Spiroplasma virus 4 (SpV4) is a bacteriophage of the Microviridae, which packages circular ssDNA within non-enveloped T = 1 icosahedral capsids. ORF1 expresses viral protein 1 (VP1), with a molecular weight of ~62 kDa, which is the major capsid protein. Lastly, VP8 encodes for an arginine–lysine-rich polypeptide that is analogous to the J-protein of phiX174 and is important for DNA packaging. A striking feature of the SpV4 capsid is the mushroom-like protrusions at the 3-fold axes, which is common among all members of the subfamily Gokushovirinae.

In this study, the capsid structures of genome-containing and empty SpV4 virions were determined to 2.5 and 3.0 Å resolution, respectively, using cryo-electron microscopy (cryo-EM) and three-dimensional (3D) image reconstruction. The observed order in the density map for the full capsids started at methionine 5 to the C-terminal isoleucine 553. An exception to the structural ordering is the surface loop at the 3-fold symmetry axis comprising aa230–291, for which only diffuse density was observed, preventing the placement of the polypeptide sequence. The SpV4 VP1 structure consists of a core, eight-stranded, anti-parallel β-barrel motif, with β-BIDG forming the inner surface of the capsid and the β-CHEF situated above β-BIDG. The EF-loop subloops are primarily situated around the 2-fold symmetry axis of the capsid surface, with the exception of the subloop EF4 that forms the mushroom-like protrusion at the 3-fold symmetry axis. The HI subloops occupy the space between the icosahedral symmetry axes, whereas the FG loop forms the channel around the 5-fold symmetry axes. The 5-fold symmetry axis showed a pore with a diameter of 4.5 Å at its narrowest point. The VP8, DNA-binding protein was observed in the interior of both genome-filled and empty SpV4 capsids. For this short, highly positively charged protein with a calculated pI of 12.9, structural order was observed for aa9–38. The N-terminal eight amino acids were not ordered but based on the first ordered residue, they should be located near the 5-fold axis. Its C-terminal phenylalanine 38 is buried inside the capsid core, in a very highly hydrophobic region near the 2-fold symmetry axis between β-CHEF, αA, and αB.

>[60x]MRRKVKNTKRHQWRLTHSARSIKRANIMPSNPRGGRRF;>[60x]MKKKMSKLNARVHDFSMFKGNHIPRSKIHIPHKTIRAFNVGEIIPIYQTPVYPGEHIKMDLTSLYRPSTFIVPPMDDLIVDTYAFAVPWRIVWKDLEKFFGENSDSWDVKNAPPVPDIVAPSGGWDYGTLADHFGITPKVPGIRVKSLRFRAYAKIINDWFRDQNLSSECALTLDSSNSQGSNGSNQVTDIQLGGKPYIANKYHDYFTSCLPAPQKGAPTTLNVGGMAPVTTKFRDVPNLSGTPLIFRDNKGRTIKTGQLGIGPVDAGFLVAQNTAQAANGERAIPSNLWADLSNATGISISDLRLAITYQHYKEMDARGGTRYVEFTLNHFGVHTADARLQRSEFLGGHSQSLLVQSVPQTSSTVEKMTPQGNLAAFSETMIQNNYLVNKTFTEHSYIIVLAVVRYKHTYQQGIEADWFRGQDKFDMYDPLLANISEQPVKNREIMVQGNSQDNEIFGFQEAWADLRFKPNSVAGVMRSSHPQSLDYWHFADHYAQLPKLSSEWLKEDYKNVDRTLALKASDNTPQLRVDFMFNTIAEKPMPLYSTPGLRRI> DDIFGELSSGKNAPKTGGGAKGNNASPAGSGNTKNNGASGADINNYAGQIKSAIESKFYDASSYAGKTCTLRIKLAPDGMLLD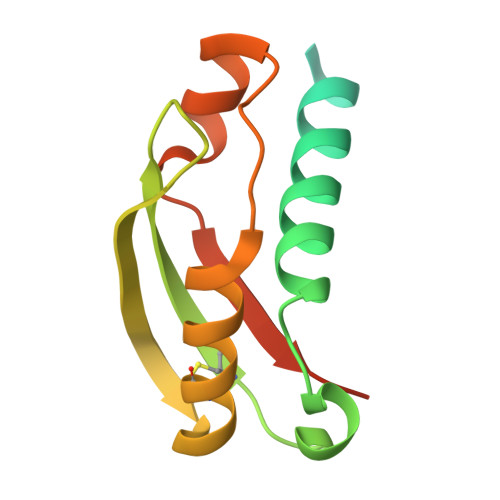IKPEGGDPALCQAALAAAKLAKIPKPPSQAVYEVFKNAPLDFKPAAAHHHHHH> AGIKVFGHPASIATRRVLIALHEKNLDFELVHVELKDGEHKKEPFLSRNPFGQVPAFEDGDLKLFESRAITQYIAHRYENQGTNLLQTDSKNISQYAIMAIGMQVEDHQFDPVASKLAFEQIFKSIYGLTTDEAVVAEEEAKLAKVLDVYEARLKEFKYLAGETFTLTDLHHIPAIQYLLGTPTKKLFT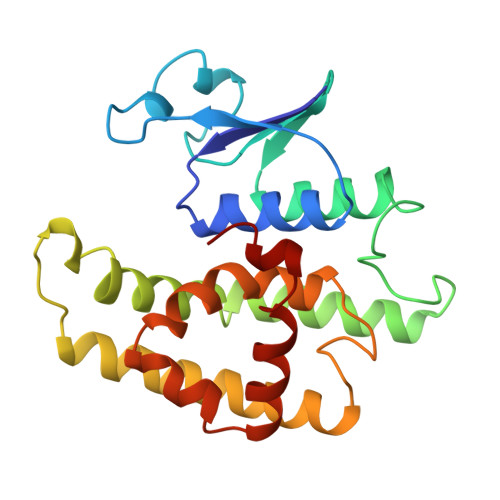ERPRVNEWVAEITKRPASEKVQ>MAKRVAIVGAGVSGLASIKCCLEEGLEPTCFERSDDLGGLWRFTEHVEEGRASLYKSVVSNSCKEMSCYSDFPFPEDYPNYVPNSQFLEYLKMYANRFNLLKHIQFKTK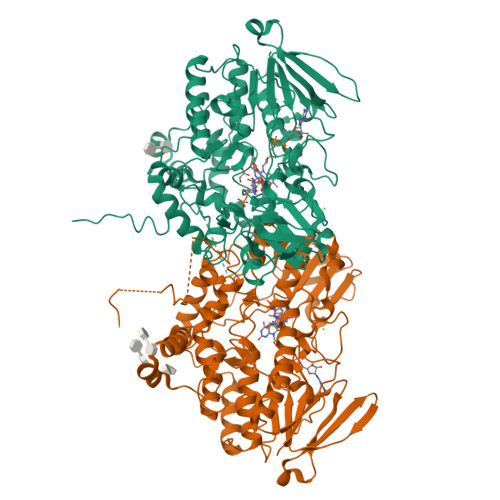VCSVTKCPDFTVTGQWEVVTQHEGKQESAIFDAVMVCTGFLTDPYLPLDSFPGINTFKGQYFHSRQYKHPDIFKDKRVLVVGMGNSGTDIAVEASHLAKKVFLSTTGGAWVMSRVFDSGYPWDMVFTTRFQNMLRNSLPTPIVTWLMARKMNSWFNHANYGLVPEDRTQLREPVLNDELPGCIITGKVLIKPSIKEVKENSVIFNNTPKEEPIDIIVFATGYTFAFPFLDESVVKVENGQASLYKYIFPAHLPKPTLAVIGLIKPLGSIIPTGETQARWAVRVLKGINKLPPQSVMIEEVNARKENKPSGFGLCYCKALQSDYITYIDELLTYINAKPNLLSMLLTDPRLALTIFFGPCTPYQFRLTGPGKWEGARNAILTQWDRTFKVTKTRIVQESPSPFASLLKLLSLPVLLLALLLMC[4x]> VSLPQSENPAFPGTLICDKDEVRIEFSSR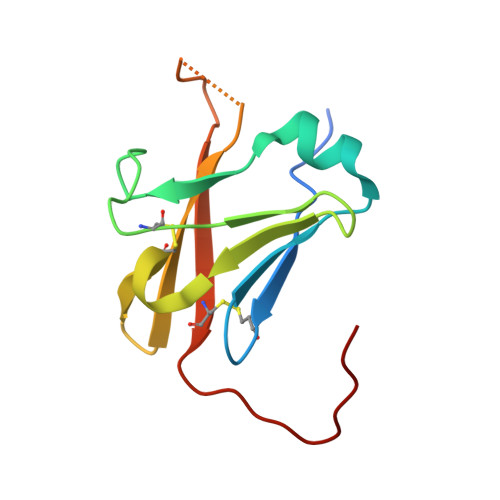FDMEKWNPSVVDTLGSEILSCTYALDLERFVLKFPYETCTIKVVGGYQVNIRVGDTTTDVRYKDDMYHFFCPAIQLEHHHHHH> MNGWNFQELKETPSQTGGPYVHIGLLPKQANIEVF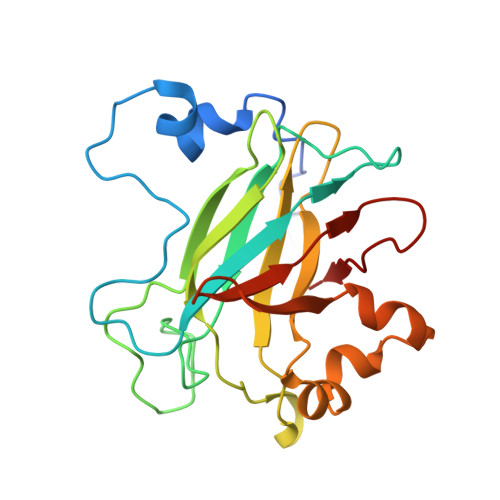EHNLDNNLVQDNTQGQRIRLEGQVFDGLSLPLRDVLIEIWQADTNGVYPSQADTQGKQVDPNFLGWGRTGADFGTGFWSFNTIKPGAVPGRKGSTQAPHISLIIFARGINIGLHTRVYFDDEAEANAKDPVLNSIEWATRRQTLVAKREERDGEVVYRFDIRIQGENETVFFDI> MIDSANRADVFLRKPAPVAPELQHEVEQFYYWEAKLLNDRRFEEWFALLAEDIHYFMPIRTTRIMRDSRLEYSGSREYAHFDDDATMMKGRLRKITSDVSWSENPASRTRHLVSNVMI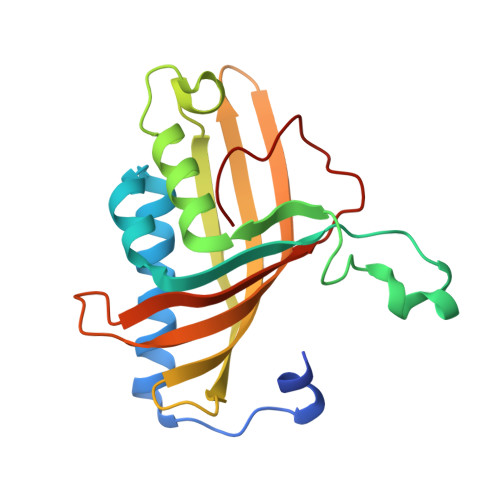VGAEAEGEYEISSAFIVYRNRLERQLDIFAGERRDTLRRNTSEAGFEIVNRTILIDQSTILANNLSFFF>MADKIKDAKIIFVVGGPGSGKGTQCEKVVAKYGYTHLSSGDLLRAEVSSGSERGKQLQAIMQKGELVPLDTVLDMIKDAMIAKADVSKGYLIDGYPREVKQGEEFEKKIGKPCLLLYIDAKGETMVKRLMKRGETSGRADDNEETIKKRLDLYYKATEPVIAFYEGR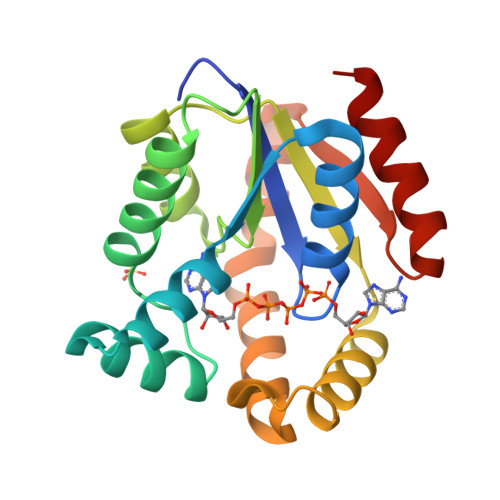GIVRKIDSELPVDEVFKQVSTAIDAL[2x]> SNAPLLLG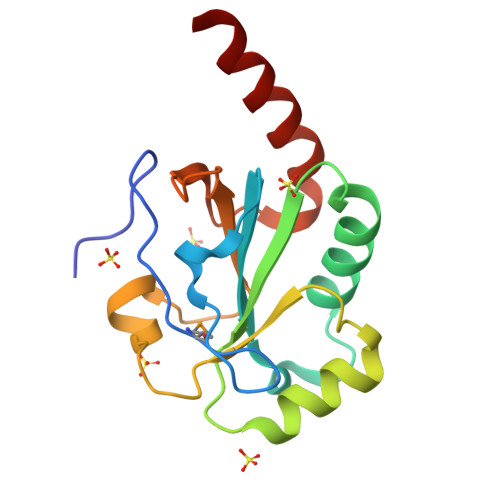KKAPNLYMTDTTGTYRYLYDVQAKYTILFFWDSQCGHCQQETPKLYDWWLKNRAKGIQVYAANIERKDEEWLKFIRSKKIGGWLNVRDSKNHTDFKITYDIYATPVLYVLDKNKVIIAKRIGYENLDDFLVQYEKSLKTK>[2x]MNLPTAQEVQGLMARYIELVDVGDIEAIVQMYADDATVED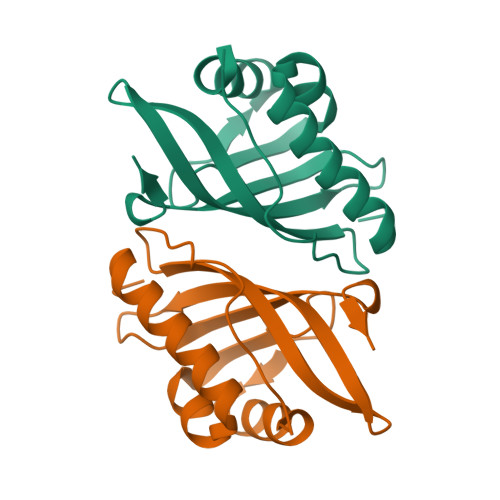PFGQPPIHGREQIAAFYRQGLGGGKVRACLTGPVRASHNGCGAMPFRVEMVWNGQPCALDVILVMRFDEHGRIQTMQAYWSEVNLSVREPQ>[2x]MSIETNTYDVIVVGSGAGAMLAAARAHDLGLSVLVV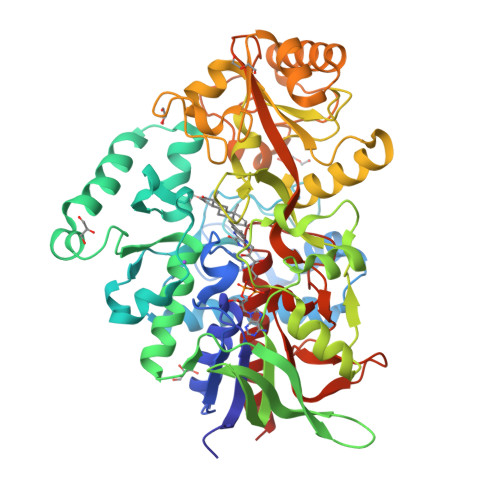EKSDKYGGTSAVSGGAVWIPNNSQMQIKDSFDEALTYLKAATQGLVAEDRLLAYLESAPQMVEYINANMTLQYFPCHRYPDYYQHLPGAKPGGRTMEPMLFDAALLGDEFANLRMAYTGTLLMGKASMTATEAHVMLAKEPGWMLQVIKSLGRYYLDLPWRLKSRHDRKRGLGNAMAAGLRHALLERKVPLWLNTPFESLITEGAENKRVTGIVVKRNGQTLQLTARRGVVLGAGGFERNQQMREQYLPKPTNAAWSATPPHNTGDTIRAAMDIGARAELMDWAWWVPSIHVPGEAAQTGLFAERNLPGCIVVNGKGQRFINEASPYLEFGAAMYENHARSGSAVPAWLIFDGKFRYNYPMGPLMPGQIQPDRKAWLGKVYWRDDTLEGLAKQIGVDAAGLKQSVELNNQYAQDGKDREFDKGGNVFDRYYGDYNVKPNPCLAPIGKPPYYAMRVDAGDIGTKGGLLTDKDARVLDESDRPIEGLYCIGNNSASVMGKAYPGAGGTLGPAMTFGFRAANHIAASK>PGGHLLNLTKPLCEVNSWHILSKDNAIRIGEDAHIIVTREPYLSCDPQGCRMFALSQGTTLRGKHANGTIHDRSPFRALVSWEMGQAPSPYNTRVECIGWSSTSC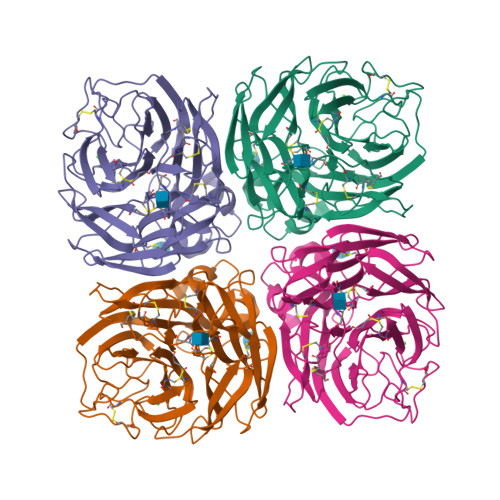HDGISRMSICISGPNNNASAVVWYGGRPVTEIPSWAGNILRTQESECVCHGGICPVVMTDGPANNRAETKIIYFKEGKIKKIEELKGDAQHIEECSCYGASEMIKCICRDNWKGANRPVITIDPEMMTHTSKYLCSKILTDTSRPNDPTNGKCEAPITGGSPDPGVKGFAFLDGENSWLGRTISKDSRSGYEMLKVPNAETDTQSGAISHQIIVNNQNWSGYSGAFIDYWANKECFNPCFYVELIRGRPKESSVLWTSNSIVALCGSKERLGSWSWHDGAEIIYFK[4x]> MTQQPLRGVTSLRFNQDQSCFCCAMETGVRIYNVEPLMEKGHLDHEQVGSMGLVEMLHRSNLLALVGGGSSPKFSEISVLIWDDAREGKDSKEKLVLEFTFTKPVLSVRMRHDKIVIVLKNRIYVYSFPDNPRKLFEFDTRDNPKGLCDLCPSLEKQLLVFPGHKCGSLQLVDLASTKPGTSSAPFTINAHQSDIACVSLNQPGTVVASASQKGTLIRLFDTQSKEKLVELRRGTDPATLYCINFSHDSSFLCASSDKGTVHIFALKDTRLNRRSALARVGKVGPMIGQYVDSQWSLASFTVPAESACICAFGRNTSKNVNSVIAICVDGTFHKYVFTPDGNCNREAFDVYLDICDDDDF;> MSRWLWPWSNCVKERVCRYLLHHYLGHFFQEHLSLDQLSLDLYKGSVALRDIHLEIWSVN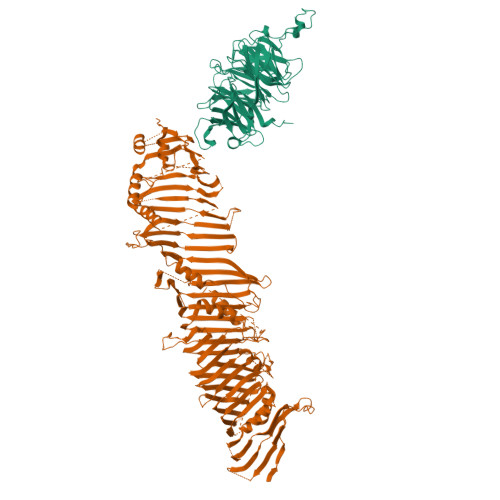EVLESMESPLELVEGFVGSIEVAVPWAALLTDHCTVRVSGLQLTLQPRRGPAPGAADSQSWASCMTTSLQLAQECLRDGLPEPSEPPQPLEGLEMFAQTIETVLRRIKVTFLDTVVRVEHSPGDGERGVAVEVRVQRLEYCDEAVRDPSQAPPVDVHQPPAFLHKLLQLAGVRLHYEELPAQEEPPEPPLQIGSCSGYMELMVKLKQNEAFPGPKLEVAGQLGSLHLLLTPRQLQQLQELLSAVSLTDHEGLADKLNKSRPLGAEDLWLIEQDLNQQLQAGAVAEPLSPDPLTNPLLNLDNTDLFFSMAGLTSSVASALSELSLSDVDLASSVRSDMASRRLSAQAHPAGKMAPNPLLDTMRPDSLLKMTLGGVTLTLLQTSAPSSGPPDLATHFFTEFDATKDGPFGSRDFHHLRPRFQRACPCSHVRLTGTAVQLSWELRTGSRGRRTTSMEVHFGQLEVLECLWPRGTSEPEYTEILTFPGTLGSQASARPCAHLRHTQILRRVPKSRPRRSVACHCHSELALDLANFQADVELGALDRLAALLRLATVPAEPPAGLLTEPLPAMEQQTVFRLSAPRATLRLRFPIADLRPEPDPWAGQAVRAEQLRLELSEPQFRSELSSGPGPPVPTHLELTCSDLHGIYEDGGKPPVPCLRVSKALDPKSTGRKYFLPQVVVTVNPQSSSTQWEVAPEKGEELELSVESPCELREPEPSPFSSKRTMYETEEMVIPGDPEEMRTFQSRTLALSRCSLEVILPSVHIFLPSKEVYESIYNRINNDLLMWEPADLLPTPDPAAQPSGFPGPSGFWHDSFKMCKSAFKLANCFDLTPDSDSDDEDAHFFSVGASGGPQAAAPEAPSLHLQSTFSTLVTVLKGRITALCETKDEGGKRLEAVHGELVLDMEHGTLFSVSQYCGQPGLGYFCLEAEKATLYHRAAVDDYPLPSHLDLPSFAPPAQLAPTIYPSEEGVTERGASGRKGQGRGPHMLSTAVRIHLDPHKNVKEFLVTLRLHKATLRHYMALPEQSWHSQLLEFLDVLDDPVLGYLPPTVITILHTHLFSCSVDYRPLYLPVRVLITAETFTLSSNIIMDTSTFLLRFILDDSALYLSDKCEVETLDLRRDYVCVLDVDLLELVIKTWKGSTEGKLSQPLFELRCSNNVVHVHSCADSCALLVNLLQYVMSTGDLHPPPRPPSPTEIAGQKLSESPASLPSCPPVETALINQRDLADALLDTERSLRELAQPSGGHLPQASPISVYLFPGERSGAPPPSPPVGGPAGSLGSCSEEKEDEREEEGDGDTLDSDEFCILDAPGLGIPPRDGEPVVTQLHPGPIVVRDGYFSRPIGSTDLLRAPAHFPVPSTRVVLREVSLVWHLYGGRDFGPHPGHRARTGLSGPRSSPSRCSGPNRPQNSWRTQGGSGRQHHVLMEIQLSKVSFQHEVYPAEPATGPAAPSQELEERPLSRQVFIVQELEVRDRLASSQINKFLYLHTSERMPRRAHSNMLTIKALHVAPTTNLGGPECCLRVSLMPLRLNVDQDALFFLKDFFTSLVAGINPVVPGETSAEARPETRAQPSSPLEGQAEGVETTGSQEAPGGGHSPSPPDQQPIYFREFRFTSEVPIWLDYHGKHVTMDQVGTFAGLLIGLAQLNCSELKLKRLCCRHGLLGVDKVLGYALNEWLQDIRKNQLPGLLGGVGPMHSVVQLFQGFRDLLWLPIEQYRKDGRLMRGLQRGAASFGSSTASAALELSNRLVQAIQATAETVYDILSPAAPVSRSLQDKRSARRLRRGQQPADLREGVAKAYDTVREGILDTAQTICDVASRGHEQKGLTGAVGGVIRQLPPTVVKPLILATEATSSLLGGMRNQIVPDAHKDHALKWRSDSAQD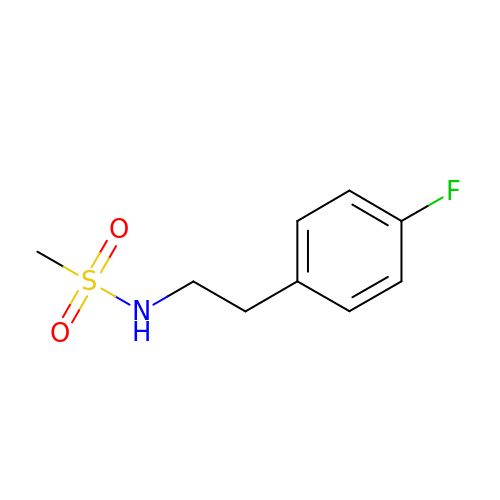~{N}-[2-(4-fluorophenyl)ethyl]methanesulfonamide | C9 H12 F N O2 S | JZUQJFQXYYHUJT-UHFFFAOYSA-N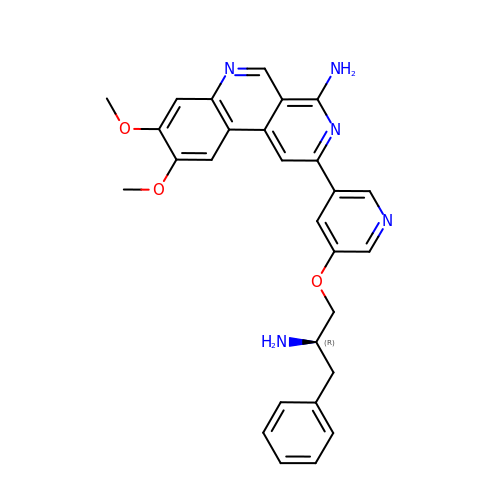2-(5-{[(2R)-2-amino-3-phenylpropyl]oxy}pyridin-3-yl)-8,9-dimethoxybenzo[c][2,7]naphthyridin-4-amine | C28 H27 N5 O3 | XNXUJUXYVTYIGP-LJQANCHMSA-N>GSHMPGFYEIVIKVPSDLDGHLPGISDSFVNWVAEKEWELPPDSDMDLNLIEQAPLTVAEKLQRDFLTEWRRVSKAPEALFFVQFEKGESYFHMHVLVETTGVKSMVLGRFLSQIREKLIQRIYRGIEPTLPNWFAVTKTRNGAGGGNKVVD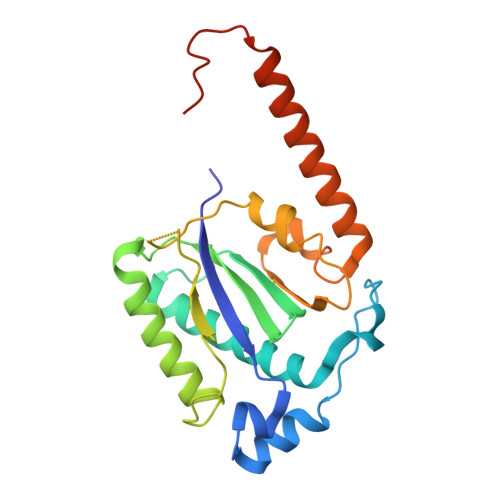ESYIPNYLLPKTQPELQWAWTNMEQYLSACLNLTERKRLVAQHLTHVSQTQEQNKENQNPNSDAPVIRSKTSARY[11x]> GAMGSLKISDNEYALIEHPGFANNKDAFFQTLGGVQSIQKACQTSFQNPAAALLELNLRPKDKYHHPVQARVQSRNDLLVTIKKMDNSVQNVSRIRQVFLFR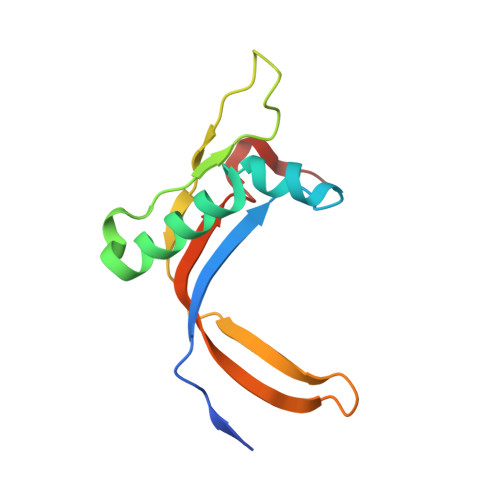DMADFQYSTQ>MIHKLADVQSQNIGDNTKVWQFCVILAGAVIGRNCNICANSLIENDVVIGDNVTIKSGVQIWDGIHIQDDVFIGPNVTFTNDKQPRSKIYPDEYLKTIVKKGASIGANSTILPGILIGENAMVGAGAVITKNVPDNAIVIGNPGRITGYVEANTGVIMPSNNFELKLQMSKVKGVSLHKFHLVNDLRGNLSVGEFEKDIPFTP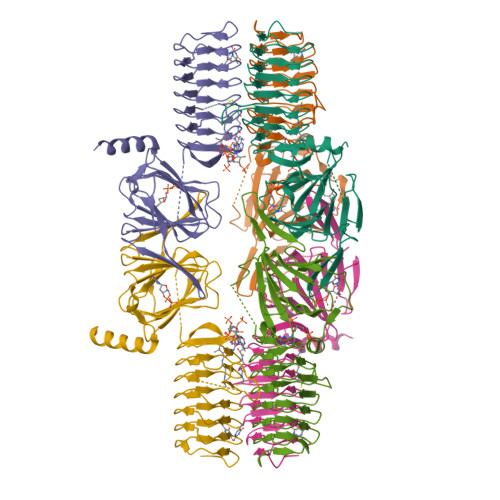KRYFTVFGVPNKEVRGEHAHKECKQFLICVSGNCSVLVDDGENREEYVLDSIDKGIYLPPMTWGVQYKYSKDAVLLVFASHYYDSDDYIRDYSTFKQMRQNLEHHHHHH[12x]>MQGCPFAKRDGTVDSSLPQKRADAPETTTFGRCAVKSNQAGGGTRSHDWWPCQLRLDVLRQFQPSQNPLGGDFDYAEAFQSLDYEAVKKDIAALMTESQDWWPADFGNYGGLFVRMAWHSAGTYRAMDGRGGGGMGQQRFAPLNSWPDNQNLDKARRLIWPIKQKYGNKISWADLMLLTGNVALENMGFKTLGFGGGRADTWQSDEAVYWGAETTFVPQGNDVRYNNSVDINARADKLEKPLAATHMGLIYVNPEGPNGTPDPAASAKDIREAFGRMGMNDTETVALIAGGHAFGKTHGAVKGSNIGPAPEAADLGMQGLGWHNSVGDGNGPNQMTSGLEVIWTKTPTKWSNGYLESLINNNWTLVESPAGAHQWEAVNGTVDYPDPFDKTKFRKATMLTSDLALINDPEYLKISQRWLEHPEELADAFAKAWFKLLHRDLGPTTRYLGPEVPKESFIWQDPLPAREGDLIDDADVDKLKAAILSTDGLDVSKLASTAMACATTYRNSDKRGGCNGARIALEPQRNWVSNNPTQLSAVLDALKKVQSDFNGSNGNKKVSLADLIVLGGTAAVEKAAKDAGVDIKVPFSAGRVDATQEQTDVTQFSYLEPQADGFRNYGRGTARARTE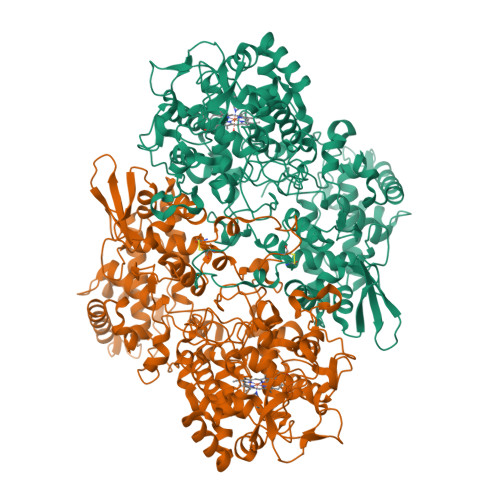EIMVDKASQLTLTPPELTVLVGGMRALGANYDGSDVGVFTANKGKLTPDFFVNLVDMNIAWTASGADGESWVGTDRKSRSEKYKGSRADLVFGSHAELRAIAEVYAENGNQEKFVKDFVAAWTKVMNLDRFDLKVKK[2x]>[2x]MLVMNTPNGNSLSAAELTCGMIMCLARQIPQATASMKD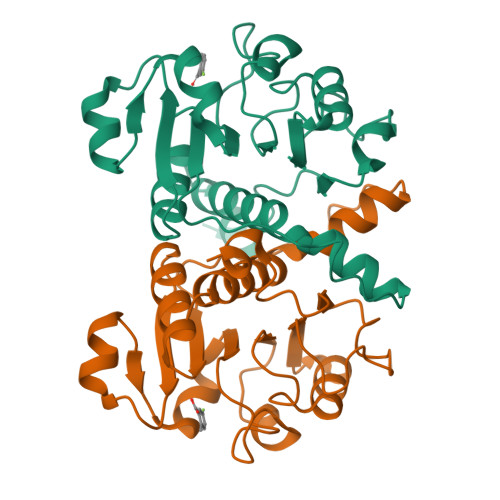GKWERKKFMGTELNGKTLGILGLGRIGREVATRMQSFGMKTIGYDPIISPEVSASFGVQQLPLEEIWPLCDFITVHTPLLPSTTGLLNDNTFAQCKKGVRVVNCARGGIVDEGALLRALQSGQCAGAALDVFTEEPPRDRALVDHENVISCPHLGASTKEAQSRCGEEIAVQFVDMVKGKSLTGV>AGPWADIMQGPSESFVDFANRLIKAVEGSNLPPSARAPVI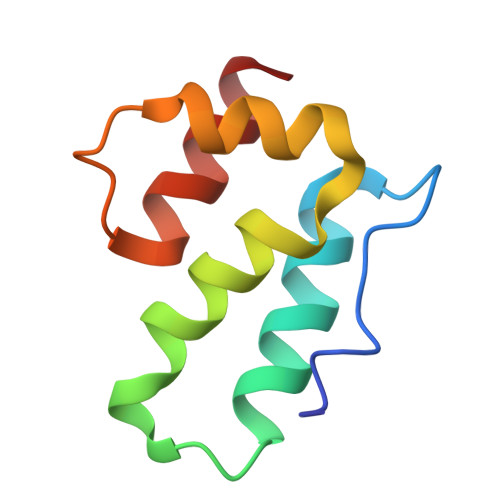IDCFRQKSQPDIQQLIRTAPSTLTTPGEIIKYVLDRQ[2x]> MVGTAHSEVNPNTRVMNSRGIWLSYVLAIGLLHIVLLSIPFVSVPVVWTLTNLIHNMGMYIFLHTVKGTPFETPD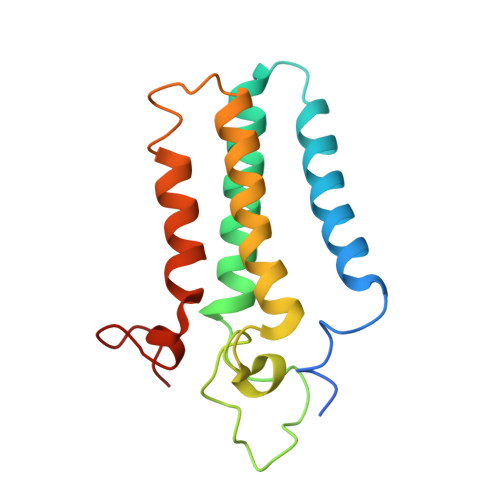QGKARLLTHWEQMDYGVQFTASRKFLTITPIVLYFLTSFYTKYDQIHFVLNTVSLMSVLIPKLPQLHGVRIFGINKY> SIRSLGYMGFAVSDVAAWRSFLTQ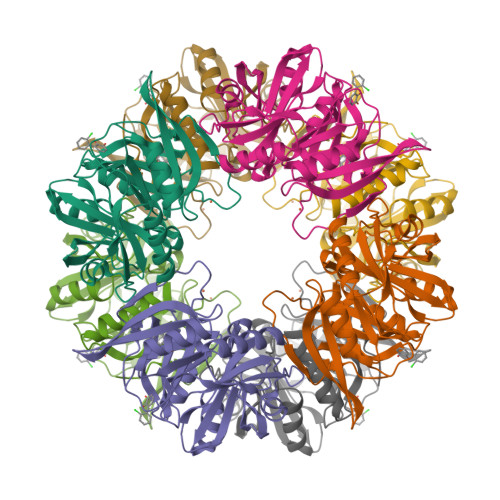KLGLMEAGTTDNGDLFRIDSRAWRIAVQQGEVDDLAFAGYEVADAAGLAQMADKLKQAGIAVTTGDASLARRRGVTGLITFADPFGLPLEIYYGASEVFEKPFLPGAAVSGFLTGEQGLGHFVRCVPDSDKALAFYTDVLGFQLSDVIDMKMGPDVTVPAYFLHCNERHHTLAIAAFPLPKRIHHFMLEVASLDDVGFAFDRVDADGLITSTLGRHTNDHMVSFYASTPSGVEVEYGWSARTVDRSWVVVRHDSPSMWGHKSVRDKAAARNKA>GMLPKGFRFGFSLAGFQSEMGLSGKDENSDWYQWCHDEYNIKNGVVSGDFPENGAAYWDLFRKDHETAVNIGMNSTRIGIEWSRIFPTSTEGVKVRIDRDGDNITGITIEKSDLESLKKICNMDAVKKYREIFMDLKDRNFYMILNLFHWSMPLWINDPRKREISKGNNLGNFFSEKSVIEFAKFAAFAAYSFDDLVDVYSTMNEPNVVFSGGNNNSEKKYYSKMKFFIEAHARAYDCIRTISRKRIGVIYANEHIESLENSDPELVEEVTWRNRYSFIDSIKSGKTFSTKNMEENSRWPEKNVFRKDLENRLDWIGVNYYSRYVVRRIESGFEAIDGYGFLCSGYEKSKDGRVVSEMGWEIYPQGLYDVLMGYQERYSLPMMVTENGIADDMDRYRPGFLISHMKMIERAIKDGAGVEGYLHWSLTDNFEWSSGFSKKFGLLRVDYRTKKRSIRPSALVFREISKKSGVPEELEWLGERFY[2x]

The genome of C. divulgatum encodes three GH1 enzyme candidates, from which CIB12 and CIB13 were heterologously expressed and characterized. Purified CIB12 and CIB13 were crystallized using the sitting-drop vapor diffusion method, and their crystal structures were determined to 2.55 Å and 2.22 Å resolution, respectively, by molecular replacement (see the section “Materials and methods” for details). Both structures revealed a classical (β/α)8 TIM-barrel fold with a spherical shape, which is typical for GH1 enzymes and is one of the most common protein folds. In the retaining catalytic mechanism of GH1 hydrolases, one of the two glutamates acts as an acid/base catalyst (Glu204 in CIB12 and CIB13) and the other acts as a nucleophile (Glu388 in CIB12 and Glu385 in CIB13). In this work, two representatives of glycosidases of GH1 family from C. divulgatum were characterized. Both CIB12 and CIB13 were active against cellobiose and lactose but showed substrate preference to cellobiose, and therefore were identified as cellobiohydrolases, EC 3.2.1.21.

In addition, the CIB12 structure contains two small antiparallel and one parallel β-sheets and six short α-helices, whereas CIB13 has four antiparallel β-sheets with two β-strands each and four α-helices outside the barrel structure. Both CIB12 and CIB13 structures revealed the presence of two protomers per asymmetric unit forming a dimer with interacting residues located primarily on two C-terminal α-helices, one side β-strand, and connecting loops. The cleavage of the glycosidic bond involves the formation of a covalent glucosyl-enzyme intermediate, which is then deglycosylated in a hydrolysis reaction via the attack of a water molecule producing the free enzyme and glucose. Both active sites show the presence of an additional area of electron density in each protomer located near the catalytic glutamates: Glu204 (3.9 Å) and Glu388 (2.8 Å) in CIB12 and Glu204 (3.5 Å) and Glu385 (2.8 Å) in CIB13. In CIB12, this density was interpreted as glycerol (two molecules in the CIB12 dimer), whereas the CIB13 dimer contained one molecule of glycerol in one protomer and one molecule of tris(hydroxymethyl)aminomethane (Tris) in the second protomer. Similarly, the Tris molecule in CIB13 was located near His148 (3.2 Å), Trp149 (3.7 Å), Tyr320 (2.6 Å), Trp423 (3.2 Å), Glu430 (3.4 Å), and Trp431 (3.2 Å). Additionally, both active sites contained several aromatic and charged residues, which might contribute to substrate binding including Gln16, Trp30, Asn203, Glu207, Tyr341, Trp362, and Phe442 in CIB12 and Gln16, Trp30, Asn203, Phe340, Met357, and Trp359 in CIB13.> MTELCPVYAPFFGAIGCASAIIFTSLGAAYGTAKSGVGICATCVLRPDLLFKNIVPVIMAGIIAIYGLVVSVLVCYSLGQKQALYTGFIQLGAGLSVGLSGLAAGFAIGIVGDAGVR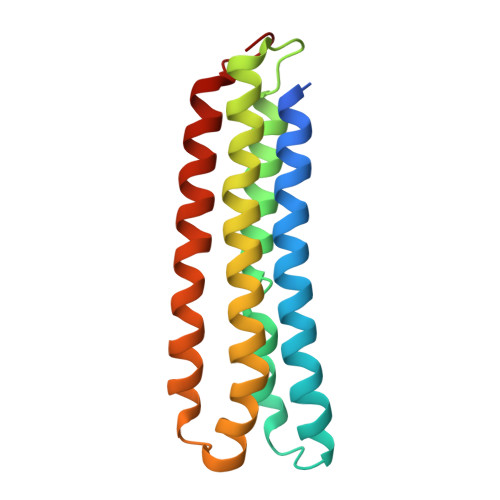GSSQQPRLFVGMILILIFAEVLGLYGLIVALLLNSRATQDVVC>[4x]MENAFKLLYKTIEERKGSPLPESYTNYLFSKGEDKILKKIG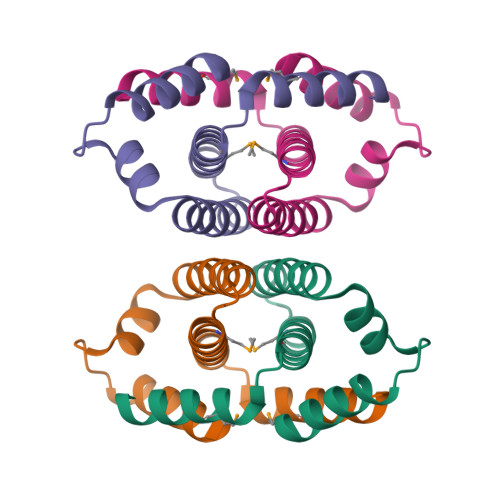EECAEVIIACKNNDKEEVVKEMVDVFYHCFVLLAEKNIALEDVMREVKERNGKLSRVGDRREIDTLLEHHHHHH> SLSSTELGDLFWSWLRDGLREGDIPVNTADACVHLTCGFVFISVPGVFFLFLKSHSRSCSSGLKESGRKEQVQA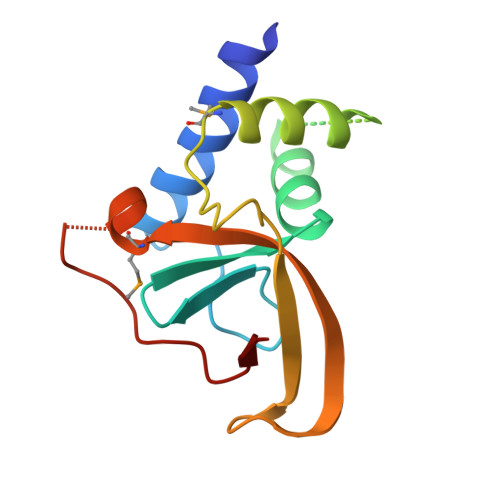AFEKMRKHRVSDSRRFWQCCLYEEPGGRGRYKKLTGYLIKMSEIYANGNFPDDSLFLKVIN TERT-BUTYL 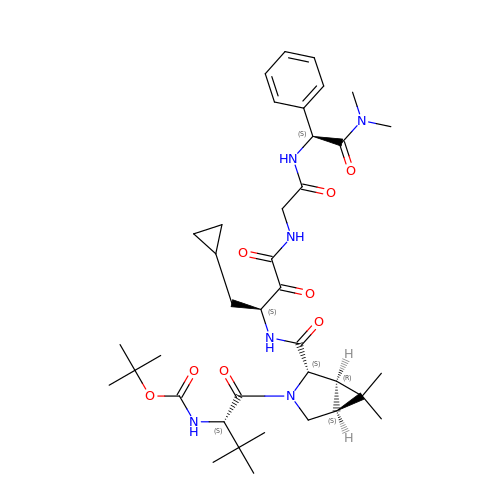[(1S)-1-({(1R,2S,5S)-2-[(3S,10S)-3-(CYCLOPROPYLMETHYL)-12-METHYL-4,5,8,11-TETRAOXO-10-PHENYL-2,6,9,12-TETRAAZATRIDECAN-1-OYL]-6,6-DIMETHYL-3-AZABICYCLO[3.1.0]HEX-3-YL}CARBONYL)-2,2-DIMETHYLPROPYL]CARBAMATE | C38 H56 N6 O8 | WHFNHDUMWYGJDL-WYFABNACSA-N>[2x]MQRIIVNPNEPYLSVIKKVVKLSIPIIVVNLLYTVENMISMILVSSISPSAVAATGFSLSLLWFIYSLMALSYSGTNILIAQFVGAKKDPSPILINGLFLSFLISLPLFFYGKDFVLFLMKVLGASETVRSLAKEYLTPIFWFIPIGFLTNTFYGAYNGAGDTKTPMKVAIIMNLTHIGTAYTLINGKFGLPKLGVEGAGWGIAISEILAFFIYTFLLIFFKKPFPLHLRLEPKLL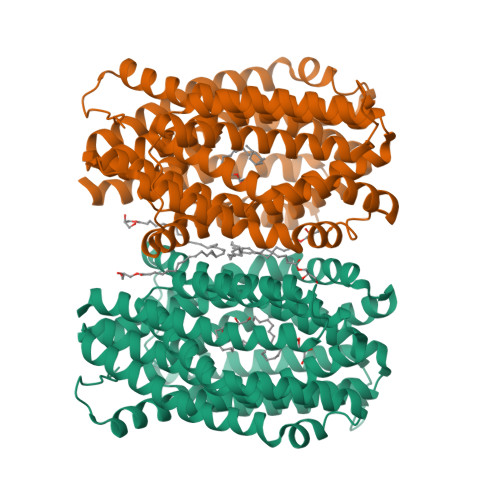FKMVRLGTPTALERAITTLSFNVFVGFLAKFGDKVLAAHQIGLRIESISFMIGFGVMIASTTLAGQNYGARNYRGMVHAVNTSAHFTALVMSLTGLILILFPHYLVYPFSRDPEVIEWASYYLQIVGISQPAMAYASIYSGALKGMGKTHIPLFVNISSFWLFRIIPSYFLLKVIHSPLVPWGFMTFETAVRALFYYTVFKKVVGKLLQTFQKEEEPEGEDAEGDKPLDEVRSKVTRNSENLYFQGGRGSHHHHHHHHHH> SEELEKALSKLSEREAMVLKMRKGLIDGREHTLEEVGA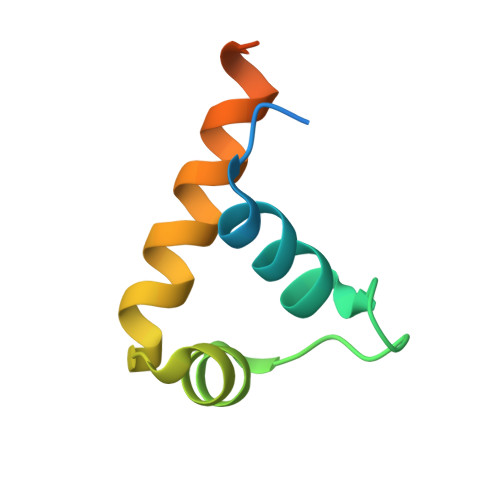YFGVTRERIRQIENKALRKLRHPSRSEKLRDFLE>ARTFFVGGNFKLNGSKQSIKEIVERLNTASIPENVEVVICPPATYLDYSVSLVKKPQVTVGAQNAYLKASGAFTGENSVDQIKDVGAKWVILGHSERRSYFHEDDKFIADKTKFALGQGVGVILCIGETLEEKKAGKTLDVVERQLNAVLEEVKDWTNVVVAYEPVWAIGTGLAAT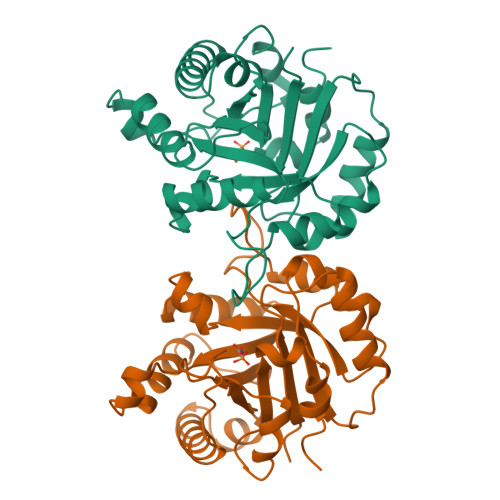PEDAQDIHASIRKFLASKLGDKAASELRILYGGSANGSNAVTFKDKADVDGFLVGGASLKPEFVDIINSRN[2x]>QLYSALANKCCHVGCTKRSLARFC[2x];>SWMEE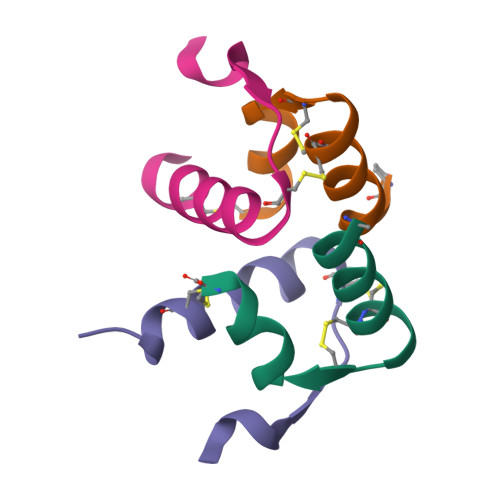VIKLCGRELVRAQIAICGMSTWS[2x]>MPTQKELRDTMSKKLQEAIKHPDPAVVAGRKSAIKRWVGVLQDNFMEHIKYFKGDKLKFLHNVFQDEGCWSGVRLDNAALGQRFTEEKIGGIDNPLRKYEMACSYCVVDKIHPLFQKRFESYRNKFPPGAFDGKTETEFGKYVRNSLLDSIKRKGPVFDFWIDRESGELKKYDAVEGFDSAVKFKWSEGVEYFYNHLKEEDKEKKLTEAILALSRVQSVEKDAPILDFCVNKIVDKDTLLQKLSQKDKGVYSLFAELIESCFFDTVHDLVQCWCYKEVSAGGDHSEKIFSQRDYELFLSSLSDTMLKNPELSVQARSLIMEFWECGSLYQYRKAAVNTSNYTVPTSGVFAELIVNWRREDIYKTDEEKEIEKKEILDMMSFAKDCFPEKFELFKKLIIRDLRLCGREGKRVNVDYGLFAEE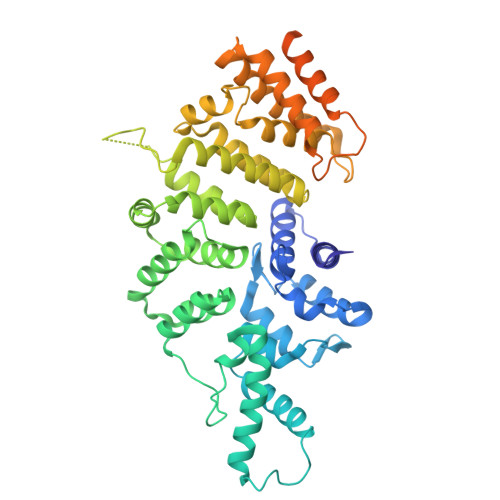LFSELEKTILPPGPVGDGPCSNLRSRSKAHGSKKTTLPVDDSPQSELGTPSVSGVSSYKKKSVFTLSGNKLEHHHHHH[2x]>[4x]MKVLALRHSVAQVYADTQIYTHDDTKDSYENAFLISNLTTHNILYFNYSARTLEILNKSGIAAIEIQSLEELFTLIRCNFTYDYENNVVYLHDYSYYTNNEIRTDQHWITKTNIEEYLLPGWKLTYVGYNGNDTRGHYNFSFTCQNAATDDDIIIEYIYSEALDFQNFMLRKIKERMTTSLPIARLSNRVFRDKLFPLLVKKHKRVVNVGPRNESMFTFLNFPSIRQFSNGPYLVKNTIKLKQERWLGKRVSQFDIGQYKNMLNVITTIYHYYNLYQEKPIIYMVGSAPSYWIYDVRQYSDFLFETWDPLDTPYSSIHHKELFFAKDIGKLKDNSILYIDIRTDRGNADWKEWRKVVELQTISNLNLAYQYLATGKSKVCCVKLTAMDLELPVSAKLLHHPTT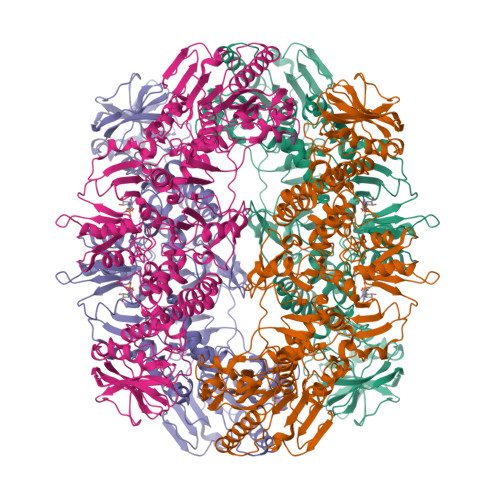EIRSEFYLLLDIWDVNNIKRFIPKGALYSFINNVITDNVFIQSPFKIRTSVSDYIVALYALSNDFNNREDIINLINNQKQSLITVRINNTFKDEPKVGFKSIYDWTFLPTDFETTNAIVTSYDGCLGIFGLSISLASKPTGNNHLFILNGTDKYYKLDQFANHTGISRRSHQVRFSESATSYSGYIFRDLSNSNFNLIGTNVENSVSGHVYNALIYYRYNYSFDLKRWIYLHSVEKANIEGGKYYEHAPIELIYACKSAKEFASLQDDLTVLRYANEIENYINKVYSITYADDPNYFIGIKFNNIPYIYDVKVPHLTFGVLYISDNMIPDVVKIMKSMKQELFGMDVTTSYTYMLSDGVYVANVSGVLATYFKMYNLFYKNQITFGQSRMFIPHITLSFSNNKTVRIETTKLRIKSIYLRKIRGDTVFDMPE> MEDIEK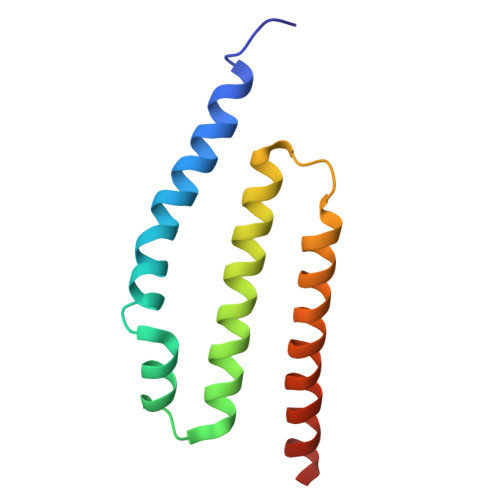IKPYVRSFSKALDELKPEIEKLTSKSLDEQLLLLSDERAKLELINRYAYVLSSLMFANMKVLGVKDMSPILGELKRVKSYMDKAKQYDNRITKSNEK>[2x]ATWTCINQQLNPKTNKW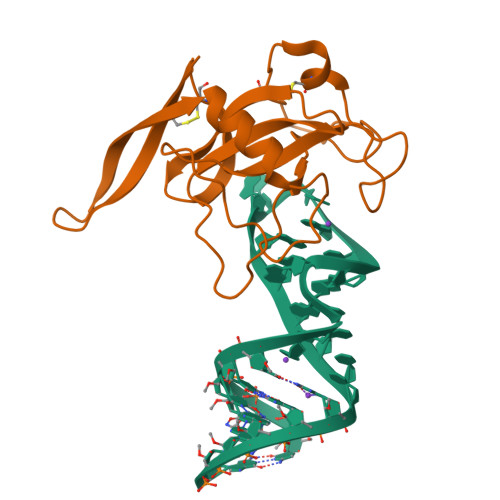EDKRLLYSQAKAESNSHHAPLSDGKTGSSYPHWFTNGYDGNGKLIKGRTPIKFGKADCDRPPKHSQNGMGKDDHYLLEFPTFPDGHDYKFDSKKPKEDPGPARVIYTYPNKVFCGIVAHQRGNQGDLRLCSH> MNDSSVIYRAIVTSKFR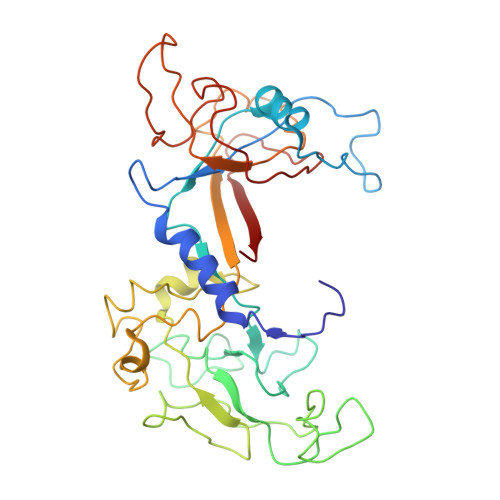TEKMLNFYNSIGSGPDKNTIFITFGRSEPWSSNENEVGFAPPYPTDSVLGVTDMWTHMMGTVKVLPSMLDAVIPRRDWGDTRYPDPYTFRINDIVVCNSAPYNATESGAGWLVYRCLDVPDTGMCSIASLTDKDECLKLGGKWTPSARSMTPPEGRGDAEGTIEPGDGYVWEYLFEIPPDVSINRCTNEYIVVPWPEELKEDPTRWGYEDNLTWQQDDFGLIYRVKANTIRFKAYLDSVYFPEAALPGNKGFRQISIITNPLEAKAHPNDPNVKAEKDYYDPEDLMRHSGEMIYMENRPPIIMAMDQTEEINILFTF>[2x]TDENLKIAIASSPAPRYITDMSIEEISREWYMLMPRQKITGGLMVKMDQAIMDKRITLKANFSVLFDQLETLVSLRAFTDDGAIVAEISPIPSMPGHSTEDVKNAIGI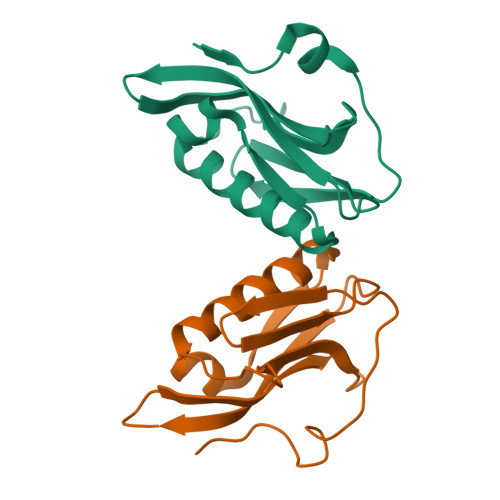LIGGLEWNDNSIRASENIQRFAWGIRDENGGPPLPPKQKRYMARRVESEV> MGHHHHHHHHHHSSGHENLYFQGHMANRNVEKLASIDAQLRLLVPGKVSEDDKLVEYDALLLDKFLDILQDLHGEDLKEAVQQCYELSAEYEGKHDPKKLEELGSLLTSLDTGDSIVIAKAFSHMLNLANLAEELQIAYRRRIKLKSGDFADEANATTESDIEETFKRLVHKLNKSPEEVFDALKNQTVELVLTAHPTQSVRRSLLQKHGRIRNCLAQLYAKDITPDDKQELDEALHREIQAAFRTDEIRRTPPTPQDEMRAGMSYFHETIWKGVPKFLRRVDTALKNIGINERFPYNAPLIQFSSWMGGDRDGNPRVTPEVTRDVCLLARMMTSNMYFSQIEDLMIEMSMWRCNSELRVRAEELYRTARKDVKHYIEFWKRIPPNQPYRVILGDVRDKLYNTRERSRHLLVDGKSDIPDEAVYTNVEQLLEPLELCYRSLCDCGDHVIADGSLLDFLRQVSTFGLSLVKLDIRQESDRHTEVLDAITQHLGIGSYREWSEEKRQEWLLAELSGKRPLIGPDLPKTEEVKDCLDTFKVLAELPSDCFGAYIISMATSTSDVLAVELLQREYHIKHPLRVVPLFEKLADLEAAPAAMTRLFSMDWYRNRIDGKQEVMIGYSDSGKDAGRFSAAWQLYKTQEQIVKIAKEFGVKLVIFHGRGGTVGRGGGPTHLALLSQPPDTINGSLRVTVQGEVIEQSFGEEHLCFRTLQRFCAATLEHGMNPPISPRPEWRELMDQMAVVATEEYRSVVFKEPRFVEYFRLATPELEFGRMNIGSRPSKRKPSGGIESLRAIPWIFSWTQTRFHLPVWLGFGAAFKHAIQKDSKNLQMLQEMYKTWPFFRVTIDLVEMVFAKGNPGIAALNDKLLVSEDLRPFGESLRANYEETKNYLLKIAGHKDLLEGDPYLKQGIRLRDPYITTLNVCQAYTLKRIRDPNYHVTLRPHISKEYAAEPSKPADELIHLNPTSEYAPGLEDTLILTMKGIAAGMQNTG;> MGHHHHHHHHHHSSGHENLYFQGHMANRNVEKLASIDAQLRLLVPGKVSEDDKLVEYDALLLDKFLDILQDLHGEDLKEAVQQCYELSAEYEGKHDPKKLEELGSLLTSLDTGDSIVIAKAFSHMLNLANLAEELQIAYRRRIKLKSGDFADEANATTESDIEETFKRLVHKLNKSPEEVFDALKNQTVELVLTAHPTQSVRRSLLQKHGRIRNCLAQLYAKDITPDDKQELDEALHREIQAAFRTDEIRRTPPTPQDEMRAGMSYFHETIWKGVPKFLRRVDTALKNIGINERFPYNAPLIQFSSWMGGDRDGNPRVTPEVTRDVCLLARMMTSNMYFSQIEDLMIEMSMWRCNSELRVRAEELYRTARKDVKHYIEFWKRIPPNQPYRVILGDVRDKLYNTRERSRHLLVDGKSDIPDEAVYTNVEQLLEPLELCYRSLCDCGDHVIADGSLLDFLRQVSTFGLSLVKLDIRQESDRHTEVLDAITQHLGIGSYREWSEEKRQEWLLAELSGKRPLIGPDLPKTEEVKDCLDTFKVLAELPSDCFGAYIISMATSTSDVLAVELLQREYHIKHPLRVVPLF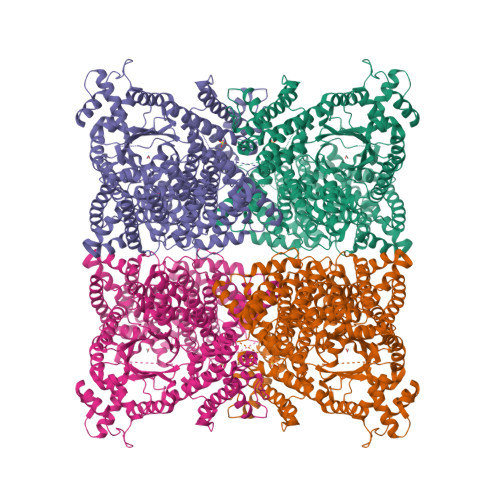EKLADLEAAPAAMTRLFSMDWYRNRIDGKQEVMIGYSDSGKDAGRFSAAWQLYKTQEQIVKIAKEFGVKLVIFHGRGGTVGRGGGPTHLALLSQPPDTINGSLRVTVQGEVIEQSFGEEHLCFRTLQRFCAATLEHGMNPPISPRPEWRELMDQMAVVATEEYRSVVFKEPRFVEYFRLATPELEFGRKNIGSRPSKRKPSGGIESLRAIPWIFSWTQTRFHLPVWLGFGAAFKHAIQKDSKNLQMLQEMYKTWPFFRVTIDLVEMVFAKGNPGIAALNDKLLVSEDLRPFGESLRANYEETKNYLLKIAGHKDLLEGDPYLKQGIRLRDPYITTLNVCQAYTLKRIRDPNYHVTLRPHISKEYAAEPSKPADELIHLNPTSEYAPGLEDTLILTMKGIAAGMQNTG> ISLGELGLLPSTVLAIGYYENFVSTVCDALHSLPTIKLNGIEYKDFVFNIIIPNDLDADIKRRAQIYFKKMDIHEVKIDTNGRSFPLYLQIDEENSGDVAVLYDMPTTLGGIDKAIEMYMKKGHIGKTSQQQLLEERELRNFKTTLINLINNNSFTKTFVKVIEE

A recent groundbreaking study discovered the ancient origins of the cGAS-STING pathway in bacteria, which play a similar role in the immune system to combat bacteriophage infections. Binding of cGG to bacterial STING causes it to oligomerize into long filaments and activates the nicotinamide adenine dinucleotide (NAD)+ cleavage activity of its fused N-terminal Toll/interleukin-1 receptor (TIR) domain. Depletion of the electron carrier NAD+ eventually leads to bacterial growth arrest or cell death, restricting the replication of invading phages in infected bacteria, a strategy called “abortive infection. In this study, we demonstrated two distinct mechanisms underlying the regulation of bacterial STINGs and a structural basis for cAA recognition and oligomerization.

To reveal the molecular mechanism underlying cAA recognition by ElSTING, we determined the 2.57 Å and 2.55 Å crystal structures of ligand-free and cAA-bound form of ElSTING, respectively, which forms canonical V-shaped dimer conformations. The ligand-binding pocket of CgSTING (~51 Å) is larger than that of ElSTING (~30 Å). CDN binding will induce the closure of the β-strand lids of CgSTING and ElSTING in nearly perpendicular directions. These structural differences result from the direction of rigid-body rotation upon ligand binding: with one protomer superimposed, the other ElSTING protomer rotated clockwise by ~26°, in contrast to the anti-clockwise rotation of CgSTING by ~21°. As a result, the ligand-binding pocket of ElSTING retains a nearly identical distance between the two stacking F169 residues; however, the distance between the two stacking residues in CgSTING is largely increased, facilitating the direct release of the ligand into the solvent upon inactivation.>MAHHHHHHAALRQPQVAELLAEARRAFREEFGAEPELAVSAPGRVNLIGEHTDYNQGLVLPMALELMTVLVGSPRKDGLVSLLTTSEGADEPQRLQFPLPTAQRSLEPGTPRWANYVKGVIQYYPAAPLPGFSAVVVSSVPLGGGLSSSASLEVATYTFLQQLCPDSGTIAARAQVCQQAEHSFAGMPCGIMDQFISLMGQKGHALLIDCRSLETSLVPLSDPKLAVLITNSNVRHSLASSEYPVRRRQCEEVARALGAASLREVQLEELEAARDLVSKEGFRRARHVVGEIRRTAQAAAALRRGDYRAFGRLMVESHRSLRDDYEVSCPELDQLVEAALAVPGVYGSRMTGGGFGGCTVTLLEASAAPHAMRHIQEHYGGTATFYLSQAADGAKVLCL[4x]

GALK1 is a small molecule kinase of the GHMP kinase family, which catalyzes the MgATP-dependent phosphorylation of the C-1 hydroxyl of α-d-galactose to yield Gal-1-P in the Leloir pathway. In classic galactosemia, GALT enzymatic deficiency causes the accumulation of Gal-1-P, the product of the enzyme galactokinase 1 (GALK1; EC 2.7.1.6) upstream of GALT in the Leloir pathway. Inhibition of human GALK1 (hGALK1) to prevent Gal-1-P production therefore could provide a therapeutic benefit for GALT deficiency. Here, we determined crystal structures of hGALK1 bound with reported ATP-competitive inhibitors of the spiro-benzoxazole series, to reveal their binding mode in the active site.

To bias hits toward allosteric binding, we soaked compounds into hGALK1 co-crystals with galactose and T2 occupying the active site. Additionally, this crystal system is biased for the detection of fragments binding to nonorthosteric sites of hGALK1 outside of the ATP and galactose pockets. hGALK1 crystals were each soaked with an individual fragment from the DSi-Poised library at a millimolar concentration. Several fragments occupy a hotspot distal from the active site ATP/galactose pockets, on the opposite face of the protein. This hotspot has not been described for any member of the GHMP kinase family and as such represents a novel pocket of unknown significance. The hotspot is a hydrophobic pocket shielded from bulk solvent by the β7−β8 loop (Pro212–Leu218). The pocket is lined on one side by strands β8– β10 (Leu218–Thr223, Tyr339–Met343 and Gly350–Ala358) and on the other side by the loop preceding β6 (Gly193–Gly196) and strands β6 and β7 (His197–Asp202 and Thr208–Val211). Fragments binding in this hotspot pocket can be classified into upper (fragments 3–6, green sticks in Figure 2C–D) and lower (fragments 7–10, blue sticks in Figure 2C,D) clusters, according to whether they extend above or below the β7−β8 loop. Fragments from the upper cluster consist of an aromatic ring separated by an amide, ester, or urea linker from another ring, which is usually aromatic (inset). One of the two constituent rings occupy the center of the pocket, stabilized by hydrophobic interactions with several residues, including Tyr300 and Phe303, which are displaced inward to do so. The linker of each fragment hydrogen bonds with residues of the β7−β8 loop and the remaining, heterocyclic, ring is more surface exposed and interacts with the side chains of Pro216 and Gln382.> WSAEDKHKEGVNSHLWIVNRAIDIMSRNTTLVKQDRVAQLNEWRTELENGIYAADTENP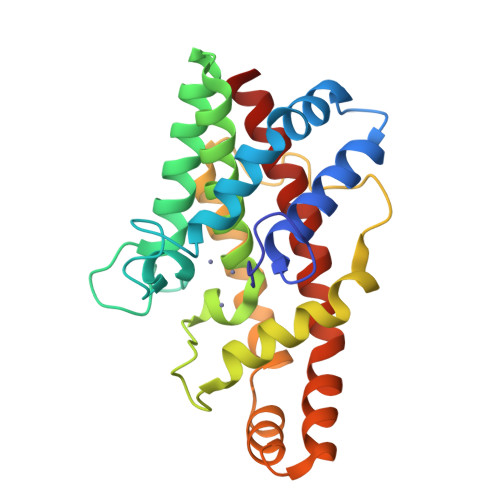YYDNSTFASHFYDPDNGKTYIPFAKQAKETGAKYFKLAGESYKNKDMKQAFFYLGLSLHYLGDVNQPMHAANFTNLSYPQGFHSKYENFVDTIKDNYKVTDGNGYWNWKGTNPEEWIHGAAVVAKQDYSGIVNDNTKDWFVKAAVSQEYADKWRAEVTPMTGKRLMDAQRVTAGYIQLWFDTYGDR CYCLO-(L-ARGININE-L-PROLINE) INHIBITOR | C11 H19 N5 O2 | 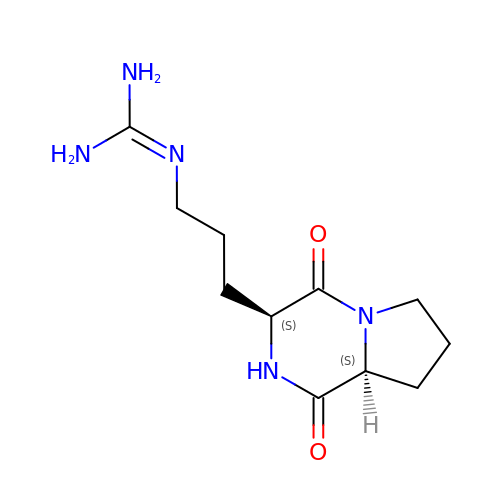ZRJHYOXNWCMGMW-YUMQZZPRSA-N>GPGSMKTRIALAQLNVTVGDFAGNVAKIVAAAQAAHDAGAHFLIAPELALSGYPPEDLLLRPAFYAASDAALAELAAQLKPFAGLAVLVGHPLRAPSADGNANRAIERGVPPVDTYNAASLIVGGEVAGTYRKQDLPNTEVFDEKRYFATDAAPYVFELNGVKFGVVICEDVWHASAAQLAK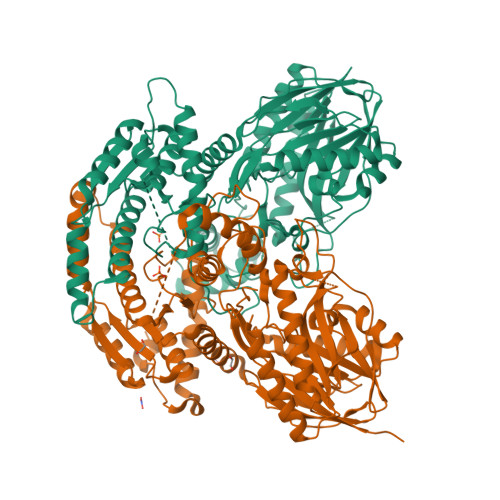AAGAQVLIVPNGSPYHMNKDAVRIDILRARIRETGLPMVYVNLVGGQDELVFDGGSFVLDGAGELVAKMPQFEEGNAIVEFDGARALPAAIAPALSVEAQVYRALVLGVRDYIGKNGFPGAIIGLSGGVDSALVLAVAVDALGAERVRAVMMPSRYTAGISTTDAADMARRVGVRYDEIAIAPMFDAFRASLAAEFAGLAEDATEENIQARIRGTLLMALSNKFGSIVLTTGNKSEMAVGYCTLYGDMAGGFAVIKDIAKTLVYRLCRYRNAAAEYGQPDIVPERILTRAPSAELRENQTDQDSLPPYDVLDAIMRMYMEEDRPLAEIVAAGYSEADVKRVTRLIKINEYKRRQAPVGIRVTHRAFGRDWRYPITSRFVESID[2x]[(3R)-3-benzylmorpholin-4-yl][5-(4-methylpyridin-2-yl)-1H-pyrazol-3-yl]methanone | C21 H22 N4 O2 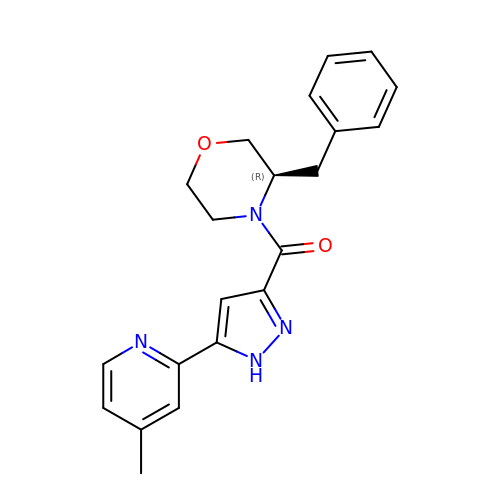| MZWBXVWTKIKBTJ-QGZVFWFLSA-N> EKHK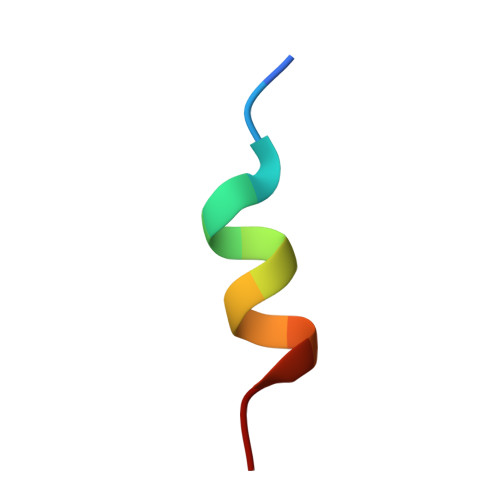ILHRLLQDS> MASMKKKGSVVIVGRINLSGDTAYAQQTRGEEGCQETSQTGRDKNQVEGEVQIVSTATQTFLATSINGVLWTVYHGAGTRTIASPKGPVTQMYTNVDKDLVGWQAPQGSRSLTPCTCGSSDLYLVTRHADVIPVRRRGDSRGSLLSPRPISYLKGSSGGPLLCPAGHAVGIFRAAVSTRGVAK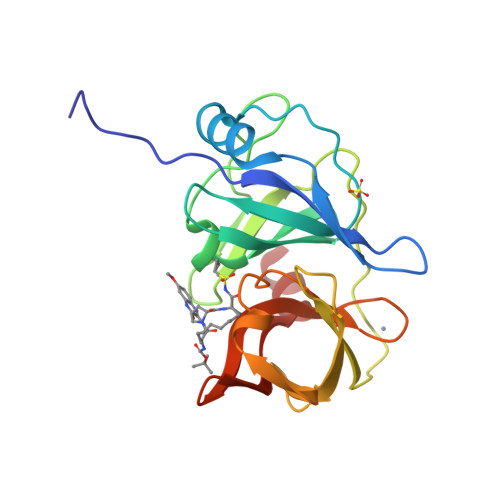AVDFIPVESLETTM> PNGQTKPLPALKLALEYIVPCMNKHGICVVDDFLGKETGQQIGDEVRALHDTGKFTDGQLVSQKSDSSKDIRGDKITWIEGKEPGCETIGLLMSSMDDLIRHCNGKLGSYKINGRTKAMVACYPGNGTGYVRHVDNPNGDGRCVTCIYYLNKDWDAKVSGGILRIFPEGKAQFADIEPKFDRLLFFWSDRRNPHEVQPAYATRYAITVWYFDADER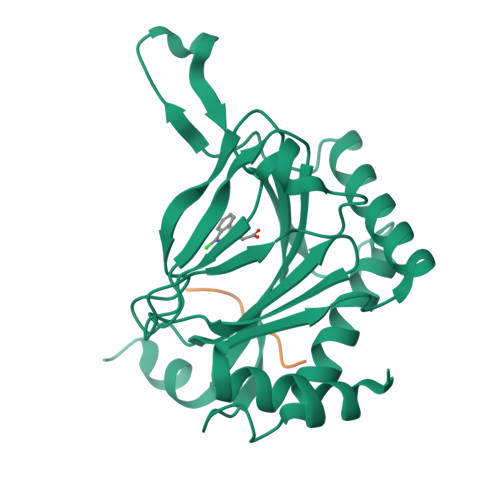ARAKVKYLTGEKGVRVELNKPSDSVGKDVF;> DLEMLAPYIPMDDDFQL>[2x]HLDCKPEFSYAIAKDERIGQLGAEGLTTTWKEYSPGMKLEDTMVIAWCEDGKLMYLQRCTRETRYLAILHTRALPTSVVFKKLFDGRKQEDVVEMDDNFEFGLCPCDAKPIVRGKFNTTLLNGPAFQMVCPIGWTGTVSCTSFNMDTLATTVVRTYRRSKPFPHRQGCITQKNLGEDLHNCILGGNWTCVPGDQLLYKGGSIESCKWCGYQFKESEGLPHYPIGKCKLENETGYRLVDSTSC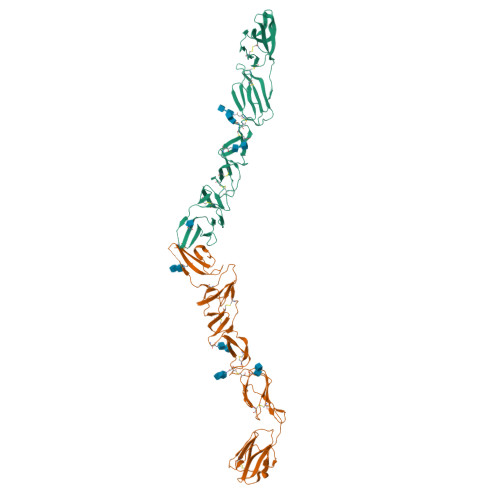NREGVAIVPQGTLKCKIGKTTVQVIAMDTKLGPMPCRPYEIISSEGPVEKTACTFNYTKTLKNKYFEPRDSYFQQYMLKGEYQYWFDLEVTDHHRD>[2x]MEDLIDGIIFAANYLGSTQLLSDKTPSKNVRMMQAQEAVSRIKMAQKLAKSRKKAP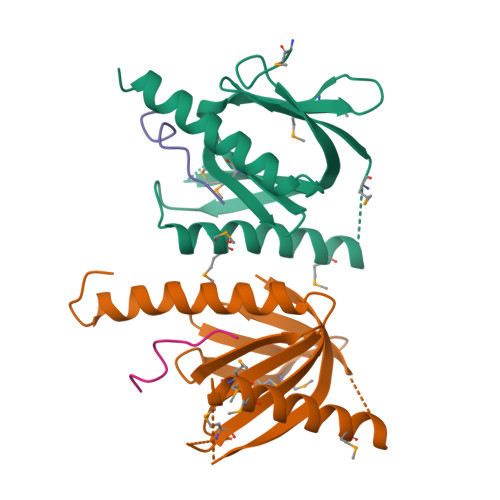EGESQPMTEVDLFILTQRIKVLNADTQETMMDHPLRTISYIADIGNIVVLMARRRIPRSNSQENVEASHPSQDGKRQYKMICHVFESEDAQLIAQSIGQAFSVAYQEFLRANGINP;>GYENPTYKFF[2x]> MGDIQVQVNIDDNGKNFDYTYTVTTESELQKVLNELMDYIKKQGAKRVRISITARTKKEAEKFAAILIKVFAELGYNDINVTFDGDTVTVEGQLEGGSLEHHHHH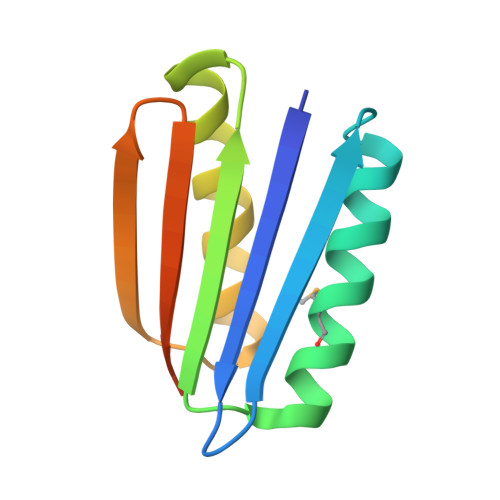H>HHMFTGSIVAIVTPMDEKGNVCRASLKKLIDYHVASGTSAIVSVGTTGESATLNHDEHADVVMMTLDLADGRIPVIAGTGANATAEAISLTQRFNDSGIVGCLTVTPYYNRPSQEGLYQHFKAIAEHTDLPQILYNVPSRTGCDLLPETVGRLAKVKNIIGIXEATGNLTRVNQIKELVSDDFVLLSGDDASALDFMQLGGHGVISVTANVAARDMAQMCKLAAEGHFAEARVINQRLMPLHNKLFVEPNPIPVKWACKELGLVATDTLRLPMTPITDSG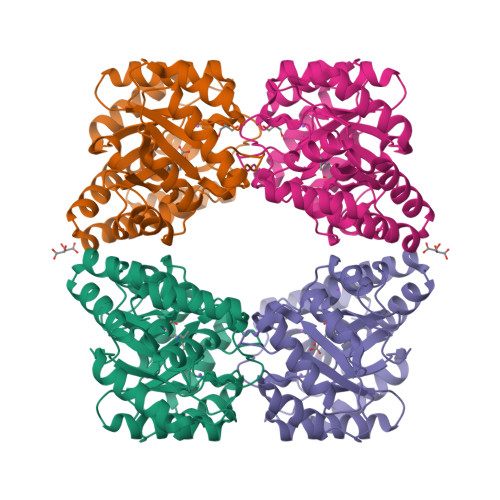RETVRAALKHAGLL[2x]4-[3-(3,5-dimethoxyphenyl)-1,2,4-oxadiazol-5-yl]-1-methyl-9-(2-methylpyridin-4-yl)-1,4,9-triazaspiro[5.5]undecane 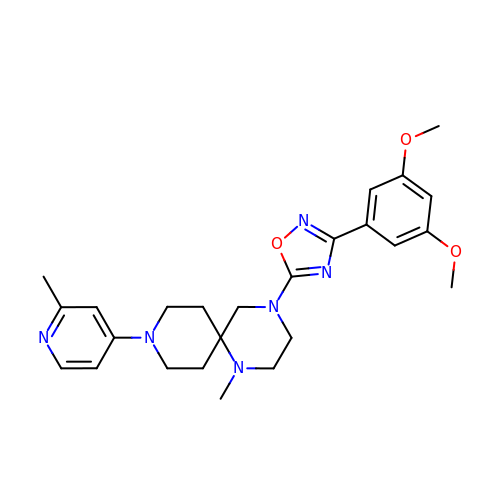| C25 H32 N6 O3 | NZYTZRHHBAJPKN-UHFFFAOYSA-N> GSARNAYLRKKIARLKKDNLQLER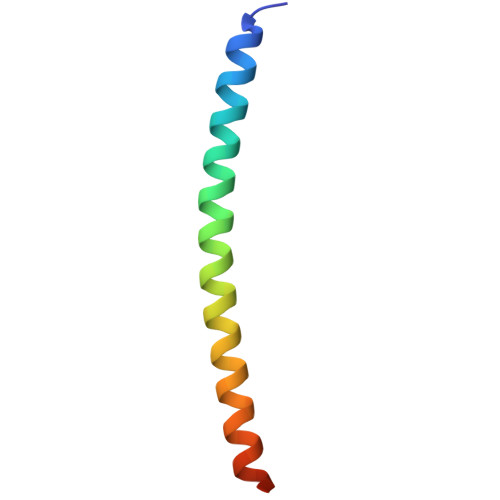DEQNLEKIIANLRDEIARLENEVASHEQ>QLDIVIVLDGSNSIYPWDSVTAFLNDLLERMDIGPKQTQVGIVQYGENVTHEFNLNKYSSTEEVLVAAKKIVQRGGRQTMTALGIDTARKEAFTEARGARRGVKKVMVIVTDGESHDNHRLKKVIQDCEDENIQRFSIAILGSYNRGNLSTEKFVE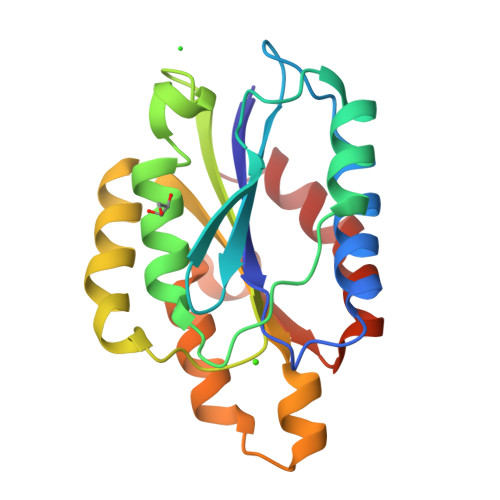EIKSIASEPTEKHFFNVSDELALVTIVKTLGERIFALEA[2x]> DLYFNPRFLADDPQAVADLSRFENGQELPPGTYRVDIYLNNGYMATRDVTFNTGDSEQGIVPCLTRAQLASMGLNTASVAGMNLLADDACVPLTTMVQDATAHLDVGQQRLNLTIPQAFMSNRARGYIPPELWDPGINAGLLNYNFSGNSVQNRIGGNSHYAYLNLQSGLNIGAWRLRDNTTWSYNSSDRSSGSKNKWQHINTWLERDIIPLRSRLTLGDGYTQGDIFDGINFRGAQLASDDNMLPDSQRGFAPVIHGIARGTAQVTIKQNGYDIYNSTVPPGPFTINDIYAAGNSGDLQVTIKEADGSTQIFTVPYSSVPLLQREGHTRYSITAGEYRSGNAQQEKPRFFQSTLLHGLPAGWTIYGGTQLADRYRAFNFGIGKNMGALGALSVDMTQANSTLPDDSQHDGQSVRFLYNKSLNESGTNIQLVGYRYSTSGYFNFADTTYSRMNGYNIETQDGVIQVKPKFTDYYNLAYNKRGKLQLTVTQQLGRTSTLYLSGSHQTYWGTSNVDEQFQAGLNTAFEDINWTLSYSLTKNAWQKGRDQMLALNVNIPFSHWLRSDSKSQWRHASASYSMSHDLNGRMTNLAGVYGTLLEDNNLSYSVQTGYAGGGDGNSGSTGYATLNYRGGYGNANIGYSHSDDIKQLYYGVSGGVLAHANGVTLGQPLNDTVVLVKAPGAKDAKVENQTGVRTDWRGYAVLPYATEYRENRVALDTNTLADNVDLDNAVANVVPTRGAIVRAEFKARVGIKLLMTLT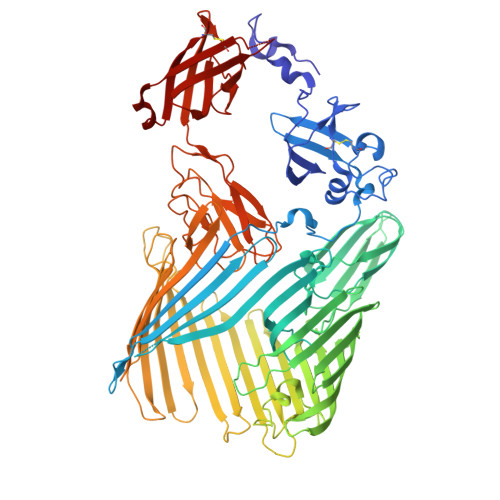HNNKPLPFGAMVTSESSQSSGIVADNGQVYLSGMPLAGKVQVKWGEEENAHCVANYQLPPESQQQLLTQLSAECR> MEKHLFNLKFAAKELSRSAKKCDKEEKAEKAKIEKAIQKGNMEVARIHAENAIRQKNQAVNFLRMSARVDAVAARVQTAVTMGKVTKSMAGVVKSMDATLKTMNLEKISALMDKFEHQFETLDVQTQQMEDTMSSTTTLTTPQ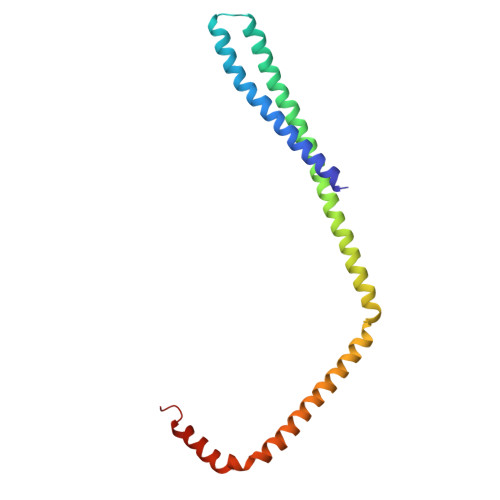NQVDMLLQEMADEAGLD> NLLSDKNVAIIGGGPVGLTMAKLLQQNGIDVSVYERDNDREARIFGGTLDLHKGSGQEAMKKAGLLQTYYDLALPMGVNIADEKGNILSTKNVKPENRFDNPEINRNDLRAILLNSLENDTVIWDRKLVMLEPGKKKWTLTFENKPSETADLVIIANGGMSKVRKFVTDTEVEETGTFNIQADIHHPEVNCPGFFQLCNGNRLMAAHQGNLLFANPNNNGALHFGISFKTPDEWKNQTQVDFQNRNSVVDFLLKEFSDWDERYKELIRVTSSFVGLATRIFPLGKSWKSKRPLPITMIGDAAHLMPPFAGQGVNSGLMDALILSDNLTNGKFNSIEEAIENYEQQMFIYGKEAQEESTQNEI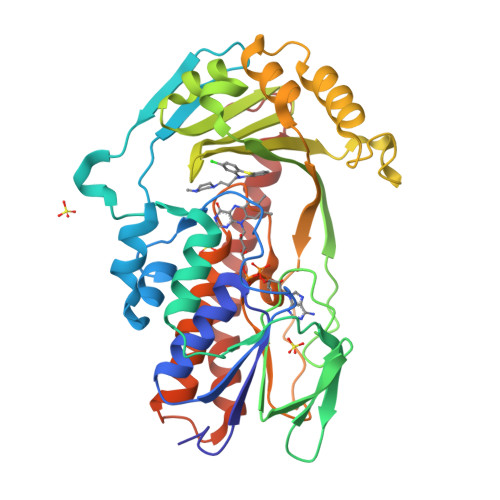EMFKPDFTF>[2x]QTKDKLEQAQNELSAWKFTPDSQTGKKLMA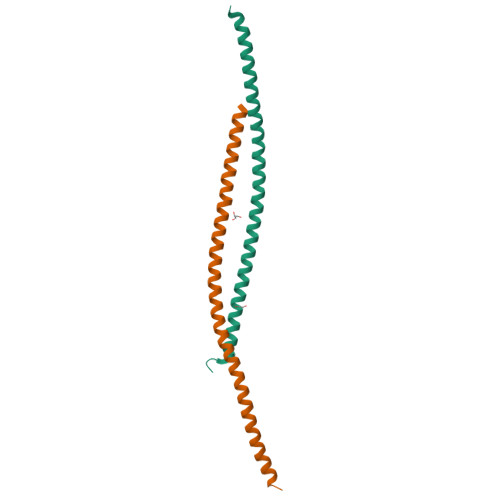KCRMLIQENQELGRQLSQGRIAQLEAELALQKKYSEELKSSQDELNDFIIQLDEEVEGMQSTILVLQQQLKETRQQLAQYQQLEHHHHHHHH>[2x]MKSRIPVVLLACGSFNPITNMHLRMFEVARDHLHQTGMYQVIQGIISPVNDTYGKKDLAASHHRVAMARLALQTSDWIRVDPWESEQAQWMETVKVLRHHHSKLLRSPPQMEGPDHGKALFSTPAAVPELKLLCGADVLKTFQTPNLWKDAHIQEIVEKFGLVCVGRVSHDPK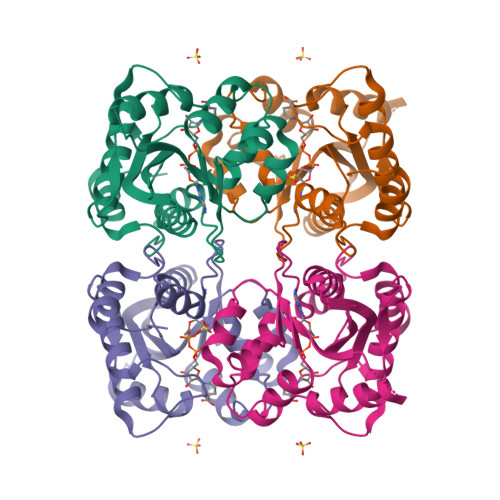GYIAESPILRMHQHNIHLAKEPVQNEISATYIRRALGQGQSVKYLIPDAVITYIKDHGLYTKGSTWKGKSTQSTEGKTS BERBERINE | C20 H18 N 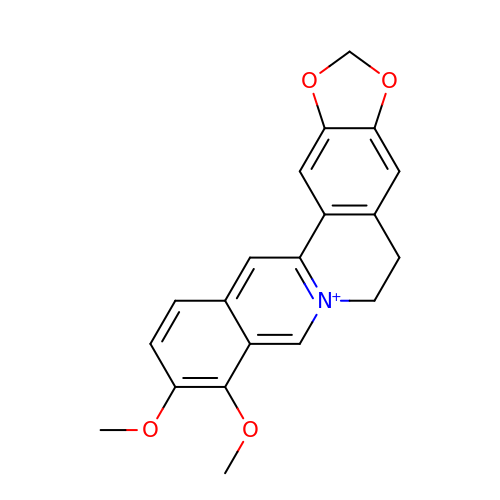O4 | YBHILYKTIRIUTE-UHFFFAOYSA-N>MIRGSTELVAIVGSPIAQVKSPQNFNTWFNHNNCNLAMLPIDLHEAALDSFADTLRGWQNLRGCVVTVPYKQALANRVDGLSERAAALGSINVIRRERDGRLLGDNVDGAGFLGAAHKHGFEPAGKRALVIGCGGVGSAIAYALAEAGIASITLCDPSTARMGAVCELLGNGFPGLTVSTQFSGLEDFDLVANASPVGMGTRAELPLSAA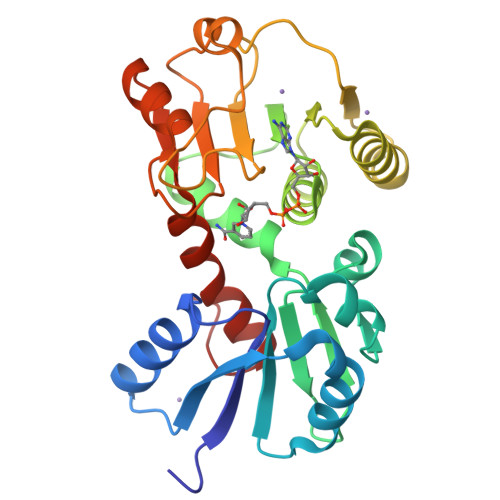LLATLQPDTLVADVVTSPEITPLLNRARQVGCRIQTGPEMAFAQLGHLGAFMGVTPLEI[2x]> MKKQNDIPQPIRGDKGATVKIPRNIERDRQNPDMLVPPETDHGTVSNMKFSFSDTHNRLEKGGYAREVTVRELPISENLASVNMRLKPGAIRELHWHKEAEWAYMIYGSARVTIVDEKGRSFIDDVGEGDLWYFPSGLPHSIQALEEGAEFLLVFDDGSFAENSTFQLTDWLAHTPKEVIAANFGVTKEEISNLPGKEKYIFENQLPGSLKDDIVEGPNGEVPYPFTYRLLEQEPIESEGGKVYIADSTNFKVSKTIASALVTVEPGAMRELHWHPNTHEWQYYISGKARMTVFASDGHARTFNYQAGDVGYVPFAMGHYVENIGDEPLVFLEIFKDDHYADVSLNQWLAMLPETF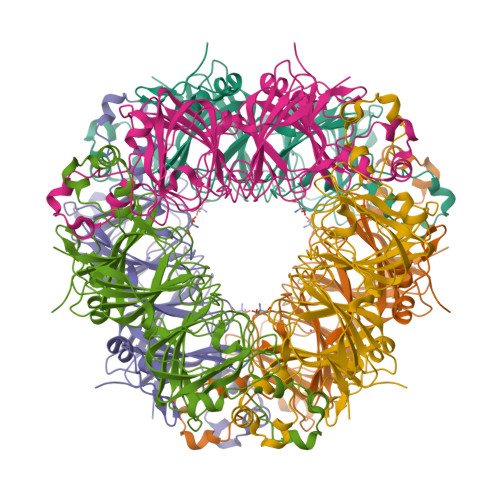VQAHLDLGKDFTDVLSKEKHPVVKKKCSK>[2x]TAPSQVLKIRRPDDWHLHLRDGDMLKTVVPYTSEIYGRAIVMPNLAPPVTTVEAAVAYRQRILDAVPAGHDFTPLM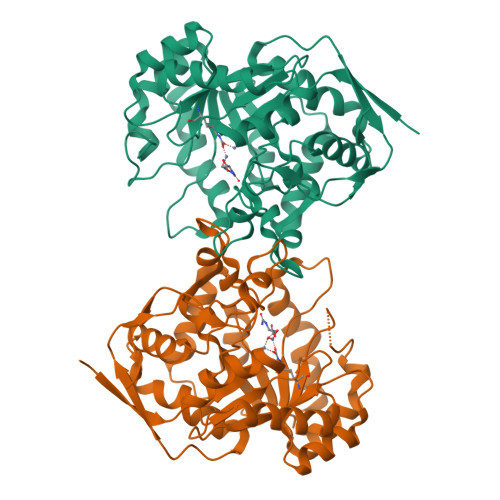TCYLTDSLDPNELERGFNEGVFTAAKLYPANATSNSSHGVTSVDAIMPVLERMEKIGMPLLVHGEVTHADIDIFDREARFIESVMEPLRQRLTALKVVFEHITTKDAADYVRDGNERLAATITPQHLMFNRNHMLVGGVRPHLYCLPILKRNIHQQALRELVASGFNRVFLGTDSAPHARHRKESSCGCAGCFNAPTALGSYATVFEEMNALQHFEAFCSVNGPQFYGLPVNDTFIELVREEQQVAESIALTDDTLVPFLAGETVRWSVKQ>HHHHHHMDPKISEMHPALRLVDPQIQLAVTRMENAVGRDQNNVGPKVYPIILRLGSPLSLNMARKTL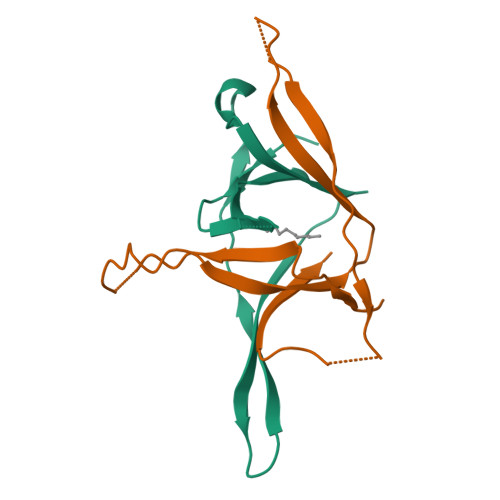NSLEDKAFQLTPIAVQMTKLATTEELPDEFVVVTVK[4x]>SNAQQQPQAFECTLVTSIETGAIINQQGACDQRVAPASTFKVPLALIG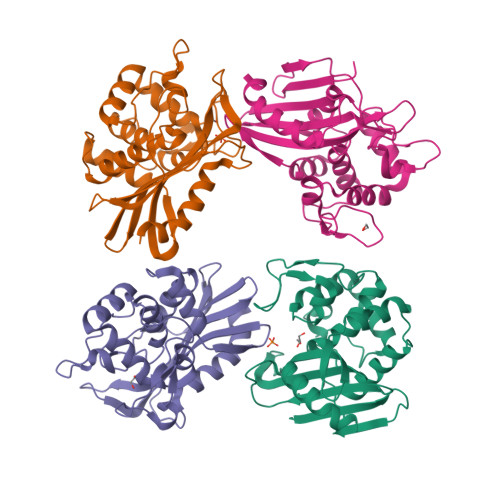FDAGILQDGKTPAWDWKPGTEARASDRKTVDPTIWEQDSVLWYSREITRRLGPEKFAAYVKRLGYGNADVSGEPGKNNGLTHSWLGASLTISPVEQVGFLRRLLGGNLPFSRDAQAKTRAIMPVFDAPESWAVHGKTGTGYMRDEKGNPDRNRPFGWFVGWAEREGQHIVFARLRVSDKPSNEPLGPAVRDAFLRDIPRLAVHR[4x]>MKLPVREFDAVVIGAGGAGMRAALQISQSGQTCALLSKVFPTRSHTVSAQGGITVALGNTHEDNWEWHMYDTVKGSDYIGDQDAIEYMCKTGPEAILELEHMGLPFSRLDDGRIYQRPFGGQSKNFGGEQAARTAAAADRTGHALLHTLYQQNLKNHTTIFSEWYALDLVKNQDGAVVGCTALCIETGEVVYFKARATVLATGGAGRIYQSTTNAHINTGDGVGMAIRAGVPVQDMEMWQFHPTGIAGAGVLVTEGCRGEGGYLLNKHGERFMERYAPNAKDLAGRDVVARSIMIEIREGRGCDGPWGPHAKLKLDHLGKEVLESRLPGILELSRTFAHVDPVKEPIPVIPTCHYMMGGIPTKVTGQALTVNEKGEDVVVPGLF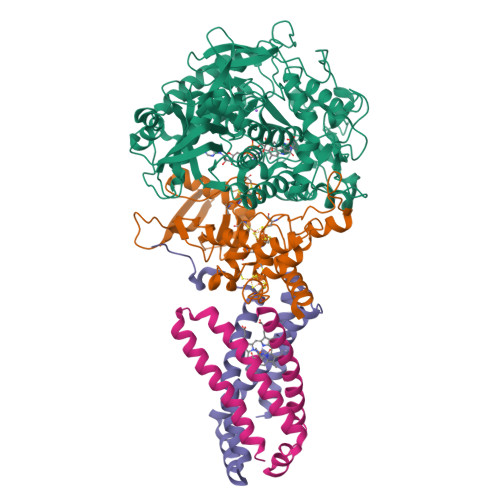AVGEIACVSVHGANRLGGNSLLDLVVFGRAAGLHLQESIAEQGALRDASESDVEASLDRLNRWNNNRNGEDPVAIRKALQECMQHNFSVFREGDAMAKGLEQLKVIRERLKNARLDDTSSEFNTQRVECLELDNLMETAYATAVSANFRTESRGAHSRFDFPDRDDENWLCHSLYLPESESMTRRSVNMEPKLRPAFPPKIRTY[3x];>[3x]MRLEFSIYRYNPDVDDAPRMQDYTLEADEGRDMMLLDALIQLKEKDPSLSFRRSCREGVCGSDGLNMNGKNGLACITPISALNQPGKKIVIRPLPGLPVIRDLVVDMGQFYAQYEKIKPYLLNNGQNPPAREHLQMPEQREKLDGLYECILCACCSTSCPSFWWNPDKFIGPAGLLAAYRFLIDSRDTETDSRLDGLSDAFSVFRCHSIMNCVSVCPKGLNPTRAIGHIKSMLLQRNA;>[3x]MIRNVKKQRPVNLDLQTIRFPITAIASILHRVSGVITFVAVGILLWLLGTSLSSPEGFEQASAIMGSFFVKFIMWGILTALAYHVVVGIRHMMMDFGYLEETFEAGKRSAKISFVITVVLSLLAGVLVW;>MVSNASALGRNGVHDFILVRATAIVLTLYIIYMVGFFATSGELTYEVWIGFFASAFTKVFTLLALFSILIHAWIGMWQVLTDYVKPLALRLMLQLVIVVALVVYVIYGFVVVWGV[3x]> MQSINFRTARGNLSEVLNNVEAGEEVEITRRGRE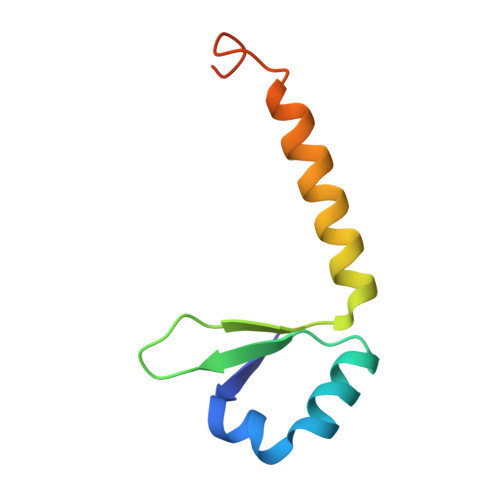PAVIVSKATFEAYKKAALDAEFASLFDTLDSTNKELVNR7-methyl-3-(1~{H}-pyrazol-4-yl)-1~{H}-indole-2-carboxylic acid 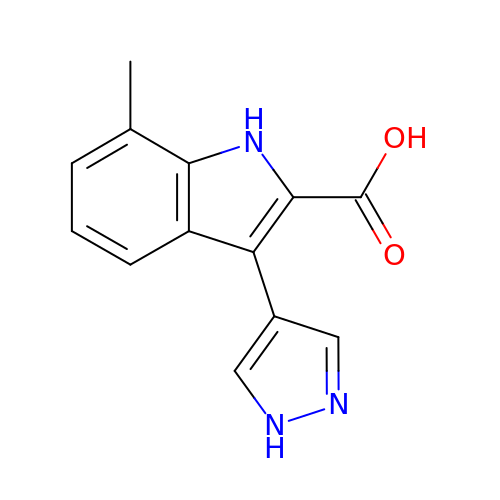| C13 H11 N3 O2 | GUEVKZFKUSZADK-UHFFFAOYSA-N>[6x]NVEEETKYIELMIVNDHLMFKKHRLSVVHTNTYAKSVVNMADLIYKDQLKTRIVLVAMETWATDNKFAISENPLITLREFMKYRRDFIKEKSDAVHLFSGSQFESSRSGAAYIGGICSLLKGGGVNEFGKTDLMAVTLAQSLAHNIGIISDKRKLASGECKCEDTWSGCIMGDTGYYLPKKFTQCNIEEYHDFLNSGGGACLFNKPSKLLDPPECGNGFIETGEECDCGTPAECVLEGAECCKKCTLTQDSQCSDGLCCKKCKFQPMGTVCREAVNDCDIRETCSGNSSQCAPNIHKMDGYSCDGVQGICFGGRCKTRDRQCKYIWGQKVTASDKYCYEKLNIEGTEKGNCGKDKDTWIQCNKRDVLCGYLLCTNIGNIPRLGELDGEITSTLVVQQGRTLNCSGGHVKLEEDVDLGYVEDGTPCGPQMMCLEHRCLPVASFNFSTCLSSKEGTICSGNGVCSNELKCVCNRHWIGSDCNTYFPHNDDAKTGITLSGKHHHHHH;>[6x]DAAQPATEFAKSQDLPYQSLSIDTFSYLNDEYVVIAQPFTGKCIFLEWDHVEKTFRNYDNITGTSTVVCKPIVIETQLYVIVAQLFGGSHIYKRDSFANKFIKIQDIEILKIRKPNDIETFKIENNWYFVVADSSKAGFTTIYKWNGNGFYSHQSLHAWYRDTDVEYLEIVRTPQTLRTPHLILSSSSQRPVIYQWNKATQLFTNQTDIPNMEDVYAVKHFSVKGDVYICLTRFIGDSKVMKWGGSSFQDIQRMPSRGSMVFQPLQINNYQYAILGSDYSFTQVYNWDAEKAKFVKFQELNVQAPRSFTHVSINKRNFLFASSFKGNTQIYKHVIVDLSAKHHHHHH

LGI1 is a 60-kDa secreted neuronal protein, which consists of the N-terminal leucine-rich repeat (LRR) domain and the C-terminal epitempin-repeat (EPTP) (also known as EAR) domain4. ADAM22 serves as a receptor for LGI1 and is anchored to the excitatory postsynaptic density through PSD-95 scaffold. The LGI1–ADAM22 ligand–receptor interaction plays an essential role in AMPA-type glutamate receptor-mediated synaptic transmission via PSD-9533–35. In this study, we present the crystal structures of LGI1 LRR, LGI1 EPTP–ADAM22, and LGI1–ADAM22 at 1.78, 2.67, and 7.13 Å resolutions, respectively.

We crystallized the complex between LGI1 EPTP and ADAM22 ECD to elucidate the mechanism of the interaction between LGI1 and ADAM22. LGI1 EPTP folds into a seven-bladed β-propeller (blades 1–7). The disulfide bond between Cys260 in blade 1 and Cys286 in blade 2 stabilizes the whole β-propeller structure. Inside the central channel, Ca2+ is coordinated by the side chains of Asp334, Glu336, and Asp381, the main-chain O atom of Val382, and a water molecule bound to Glu383. The metalloprotease-like domain of ADAM22 binds to the EPTP domain of LGI1 with a buried surface area of 1034 Å2. Trp398, Tyr408, and Tyr409 of ADAM22 are stacked in layer and project into the inner rim of the central channel of LGI1 EPTP to interact hydrophobically with Phe256, Val284, Leu302, Tyr433, and Met477 of LGI1. In addition, four hydrogen bonds are formed between LGI1 and ADAM22: Arg330 and Lys331 of LGI1 hydrogen bond with the side and main chains of Asp405 of ADAM22, respectively, and Lys353 and Arg378 of LGI1 hydrogen bond with Glu359 of ADAM22. In our pull-down analyses, the W398D, Y408A, Y409A, or Y408A Y409A mutation of ADAM22 almost or completely abolished its binding to LGI1, indicating that the hydrophobic interaction mediated by Trp398, Tyr408, and Tyr409 of ADAM22 is essential for binding between LGI1 and ADAM22. The disulfide bond between Cys394 and Cys401 tethers the N- and C-terminal ends of the Trp398-containing loop to support its conformational change.> SPTVEECGYSDRVRSITLGNSTITTQECANVVVGYGVWP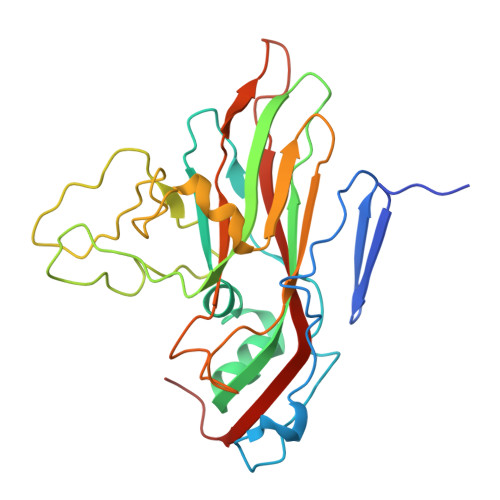DYLKDNEATAEDQPTQPDVATCRFYTLDSVQWQKTSPGWWWKLPDALSNLGLFGQNMQYHYLGRTGYTIHVQCNASKFHQGCLLVVCVPEAEMGCATLDNTPSSAELLGGDAAKEFAGEPIASGSNKLVQRVVYNAGMGIGVGNLTIFPHQWINLRTNNSATIVMPYTNSVPMDNMFRHNNVTLMVIPFVPLDYCPGSTTYVPITVTIAPMNAEYNGLRLAGHQ> NATRQLEWD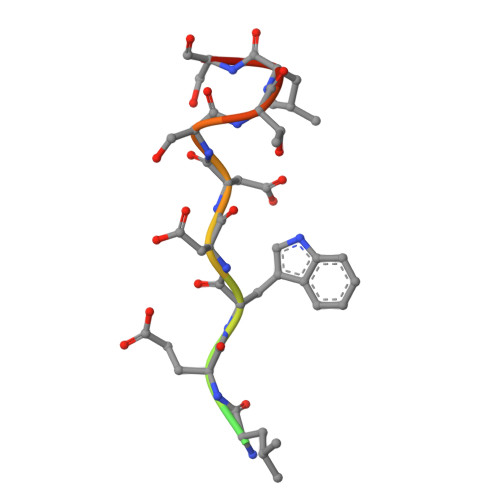DSTLSY> AGHMLPVEPPAELLQLGGGDVGGGRLSVDASDIAEASRDFGGVARAEPMAVFHPRAAGDVAGLVGAAFRSARGFRVSARGHGHSISGQAQAAGGVVVDMSRGRGPGAAVARALPVHSAALGGHYVDVWGGELWVDVLNWTLSHGGLAPRSWTDYLYLSVGGTLSNAGISGQAFHHGPQISNVYELDVVTGKGEVVTCSETENPDLFFGVLGGLGQFGIIT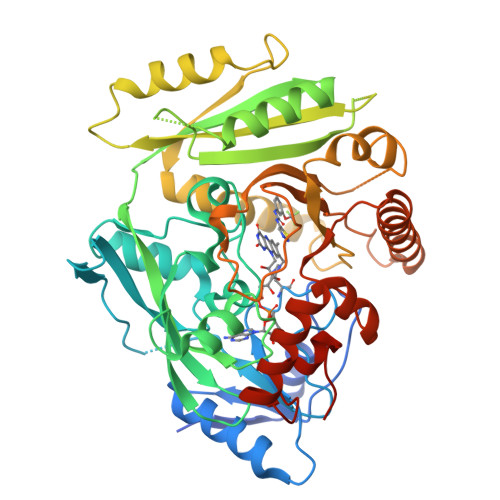RARIALERAPKRVRWIRALYSNFSEFTADQERLISLGSGGGRRFDYVEGFVVAAEGLINNWRSSFFSPQNPVKLTSLKHHSSVLYCLEVTKNYDDETAGSVDQDVDTLLGELNFLPGTVFTTDLPYVDFLDRVHKAELKLRAKGMWEVPHPWLNLFVPASRIADFDRGVFRGVLGGRTAGAGGPVLIYPMNKHKWDPRSSAVTPDEEVFYLVAFLRSALPGAPESLEALARQNQRILDFCAGTGIGAKQYLPGHKARHEWAEHFGAARWDRFARLKAEFDPRAILAAGQGIFRPPGSPALAADS> METVQDCENKLPPSLKSRLCEIRRYEIIEGPEMDKHIHCVMRALDFVYEDGRGD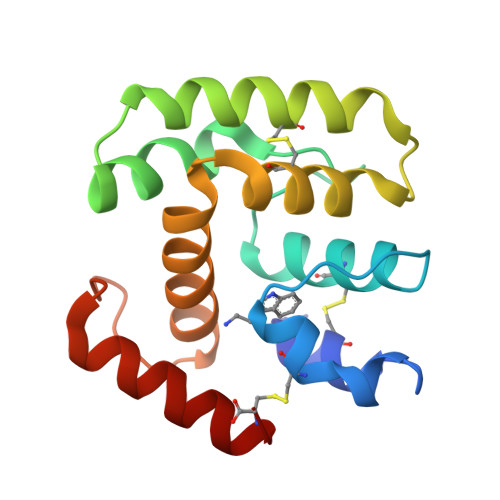YHKLYDPLNIIELDKRHDVNLEKCIGECVQVPTSERAHVFYKCLLKSTTGRTFKKVFDLMELKKAGKVPQHQRYTAEFVQIMKDYDKALNC>GSVIDPSELTFVQEIGSGQFGLVHLGYWLNKDKVAIKTIREGAMSEEDFIEEAEVMMKLSHPKLVQLYGVCLEQAPICLVFEFMEHGCLSDYLRTQRGLFAAETLLGMCLDVCEGMAYLEEASVIHRDLAARNCLVGENQVIKVSDFGMTRFVLDDQYTSSTGTKFPVKWASPEVFSFSRYSSKSDVWSFGVLMWEVFSEGKIPYENRSNSEVVEDISTGFRLYKPRLASTHVYQIMNHCWKERPED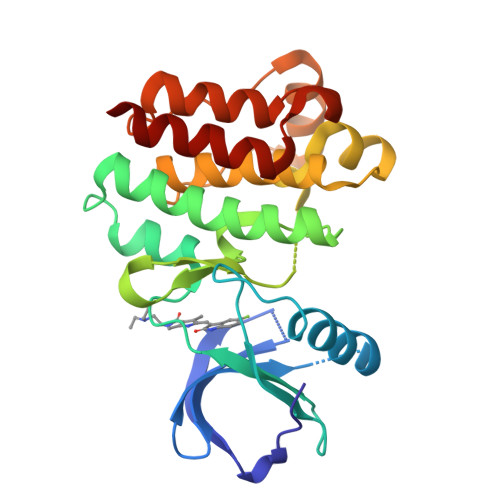RPAFSRLLRQLAAIAASGL[2x]8-hydroxyquinoline-5-carboxylic acid 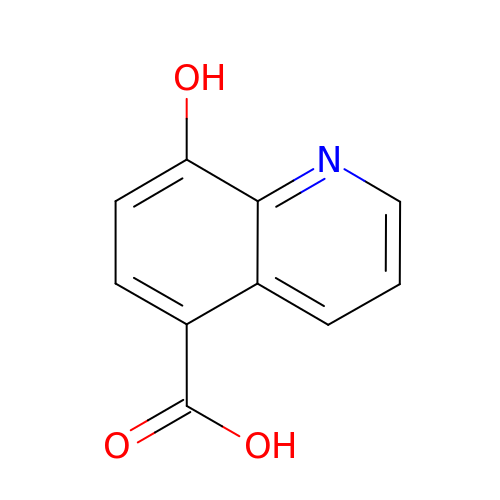| C10 H7 N O3 | JGRPKOGHYBAVMW-UHFFFAOYSA-N> GHMGKPYISAKDLKEIMYDHLPGFGTAFHQLVQVICKIGKDNNLLDTIHAEFQASLADGDSPQCALIQITKR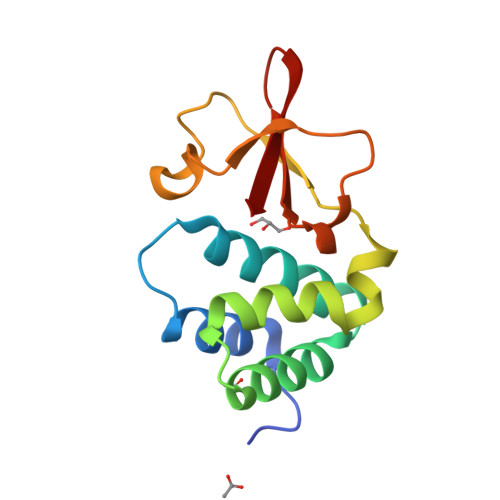VPIFQDVPPPIIHIRSRGDIPRACQKSLRPAPPSPKIDRGWVCLFKMQDGKTLGLKI> SSYAFNNGNGATNLNKSGGKKFILELIETVYEEILDLEANLRNGQQTDSTAMWEALHIDDSSYDVNPFISMLSFDKGIKIMPRIFNFLDKQQKLKILQKIFNELSHLQIIILSSYKTTPKPTLTQLKKVDLFQMIILKIIVSFLSNNSNFIEIMGLLLQLIRNNNVSFLTTSKIGLNLITILISRAALIKQDSSRSNILSSPEISTWNEIYDKLFTSLESKIQLIFPPREYNDHIMRLQNDKFMDEA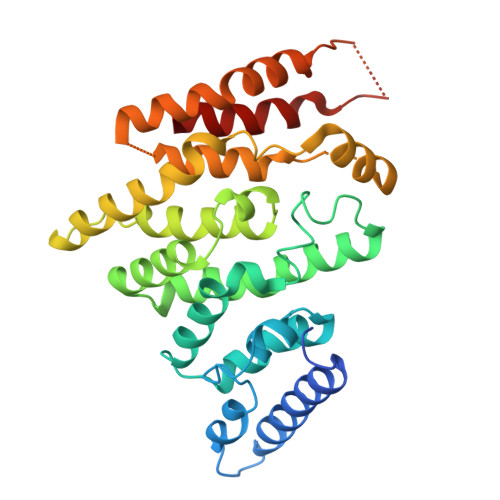YIWQFLASLALSGKLNHQRIIIDEVRDEIFATINEAETLQKKEKELSVLPQRSQELDTELKSIIYNKEKLYQDLNLFLNVM>[2x]AHHHHHHGSEYTIVDGEEYIEEIKKLDREISYSFVRFPISYEEYEERHEELFESLLSQGEHKFFVALNERSELLGHVWICITLDTVDYVKIAYIYDIEVVKWARGLGIGS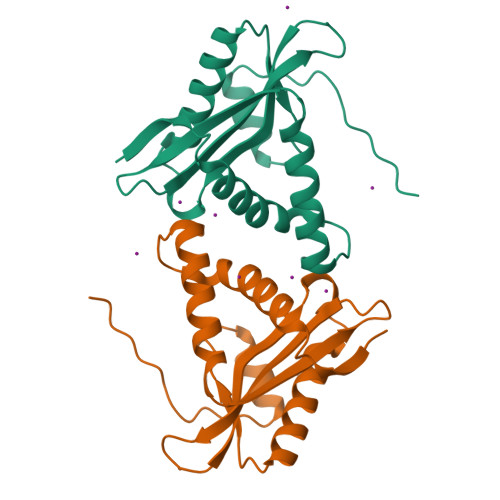ALLRKAEEWAKERGAKKIVLRVEIDNPAVKWYEERGYKARALIMEKPI> MKVLPKLALANLVCFTTLSVFAQPADPSGQQTSTNTSNLVTYLTNLGKYLGYDITQSSKAPNPPYSQLFNSNVVQLVQNYAYNTFLGAIPVDAMSQSLMNFVTDKVQGNSLINNLANTTFKYQNFSAPSSGADGKITANGLIDQSTASAQTPTTPGIFSAPQITTSGTYLNDPVSQAVFNILGTPDYSFCMDNEQKNWLPNCNLMYQNLVMQNVIGTLPPAQTSGSTPAFYSYKYNQPLISQLNSNSLIAPLLMDTSASQSGQDSGLTAKSQAQQALNFIRYASAQVTPPSLPKLSAYSELWNQATAKPNSAGYNEVQQKQAAATLSSYFNNLRVYAAQTSVGVSNLYYILSKRLPQNMSADQSNANITSQALNEFNMATRRLFDPTASNTPGQPNQQWIKQINDASPATVQKEIAILLAEINYQMYLDRQ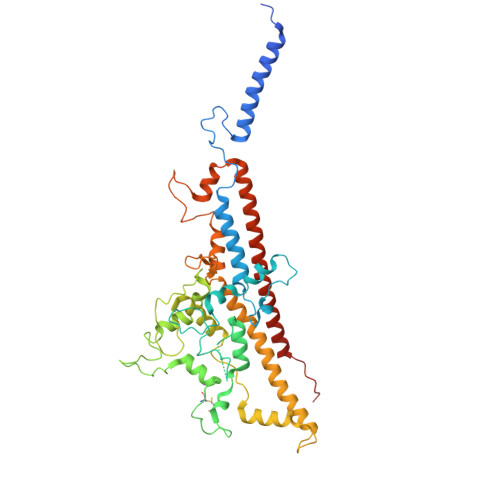IQERILLTNSIMLLQNLKAAQPTADFSSQGSPSEQ>GMSEDHPLDRPVWNSLGGPQSELDVASGNLRRLDPAYGPFAAAAPGAEAGLASLLQGDADEIWLVEPEPVAPPPGTRVIRVAPLLQMIADGPVPSFDDPGIVALGETDVPEMTALALATEPGPWASGTWRYGQFYGVRIDGRLAAMAGERMRPAPNLAEVSGVCTWPEYRGRGLAARLIRKVIAGMAARGEVPYLHSYASNASAIRLYESLGFRARRAMTATLLG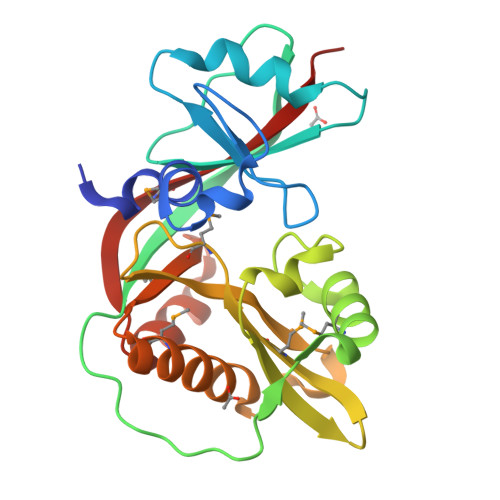KST[2x]> MDTSMKEKVKAKLVEIRKFVPFIRRVRIDFQDTLSK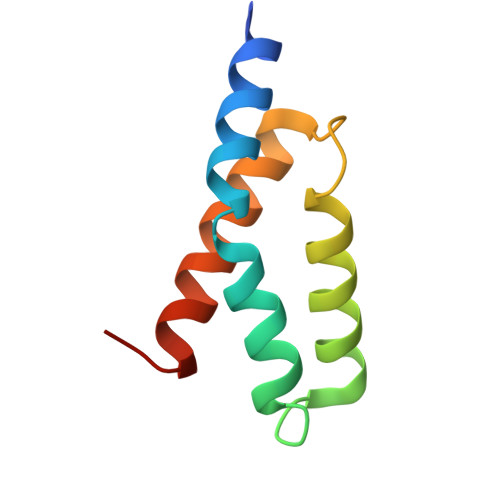VQGHRLDALVNLLDREDVSMSSLNKIEVIIDKLRTRFNPRIE N-{5-[difluoro(phosphono)methyl]-1-benzothiophene-2-carbonyl}-3-methyl-L-valyl-L-prolyl-N~3~-(4-bromophenyl)-N,N-dimethyl-beta-alaninamide | C32 H38 Br F2 N4 O7 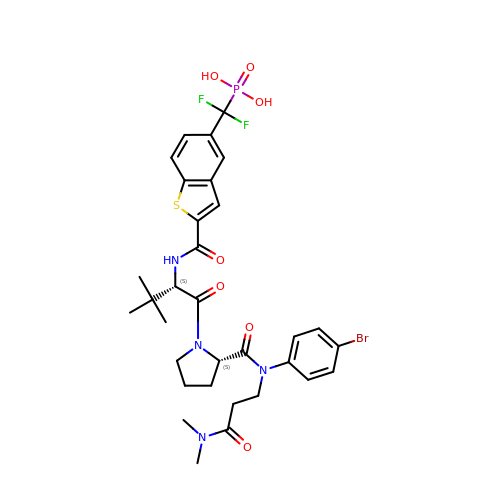P S | QHZWEMYLRQTCHK-WNCULLNHSA-N> MKKRRTFLLFSFTFLLLLSLSKADSDGDLSAMLSLKKSLNPPSSFGWSDPDPCKWTHIVCTGTKRVTRIQIGHSGLQGTLSPDLRNLSELERLELQWNNISGPVPSLSGLASLQVLMLSNNNFDSIPSDVFQGLTSLQSVEIDNNPFKSWEIPESLRNASALQNFSANSANVSGSLPGFLGPDEFPGLSILHLAFNNLEGELPMSLAGSQVQSLWLNGQKLTGDITVLQNMTGLKEVWLHSNKFSGPLPDFSGLKELESLSLRDNSFTGPVPASLLSLESLKVVNLTNNHLQGPVPVFKSSVSVDLDKDSNSFCLSSPGECDPRVKSLLLIASSFDYPPRLAESWKGNDPCTNWIGIACSNGNITVISLEKMELTGTISPEFGAIKSLQRIILGIN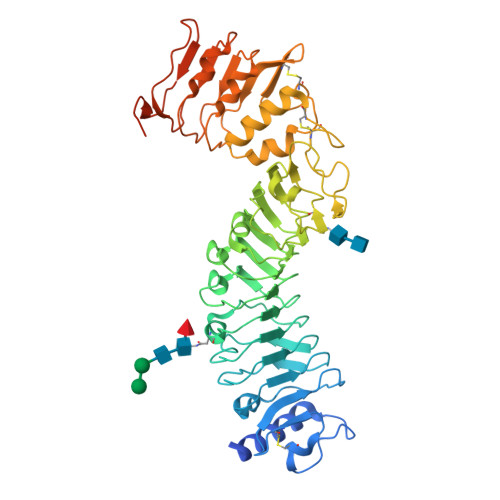NLTGMIPQELTTLPNLKTLDVSSNKLFGKVPGFRSNVVVNTNGNPDIGKDKSSLSSPGSSSPSGGSGSGINGDHHHHHH>[2x]EDICFIAGIGDTNGYGW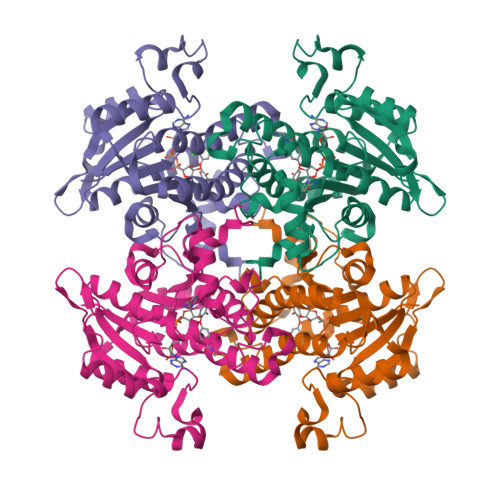GIAKELSKRNVKIIFGIWPPVYNIFMKNYKNGKFDNDMIIDKDKKMNILDMLPFDASFDTANDIDEETKNNKRYNMLQNYTIEDVANLIHQKYGKINMLVHSLANAKEVQKDLLNTSRKGYLDALSKSSYSLISLCKYFVNIMKPQSSIISLTYHASQKVVPGYGGGMSSAKAALESDTRVLAYHLGRNYNIRINTISAGPLKSRAATAINKLNNTYENNTNQNKNRNSHDVHNIMNNSGEKEEKKNSASQNYTFIDYAIEYSEKYAPLRQKLLSTDIGSVASFLLSRESRAITGQTIYVDNGLNIMFLPDDIYRNENE> GSDDGAFGDIWAYMSEALTGAPGKIIACGMLFSVAYFGVVKPNLG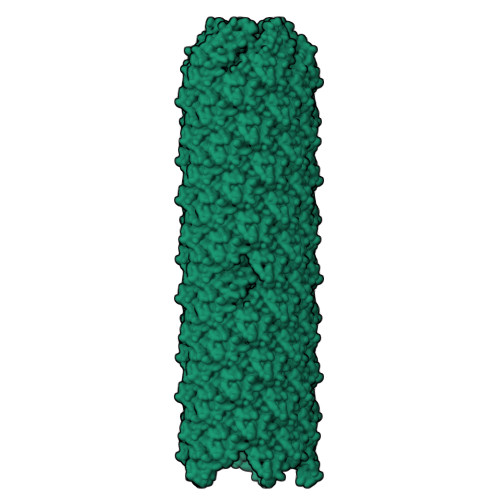LALVSALMMLVMANGEKIISSFLGAGIPL> MQGSVTEFLKPRLVDIEQVSSTHAKVTLEPLERGFGHTLGNALRRILLSSMPGCAVTEVEIDGVLHEYSTKEGVQEDILEILLNLKGLAVRVQGKDEVILTLNKSGIGPVTAADITHDGDVEI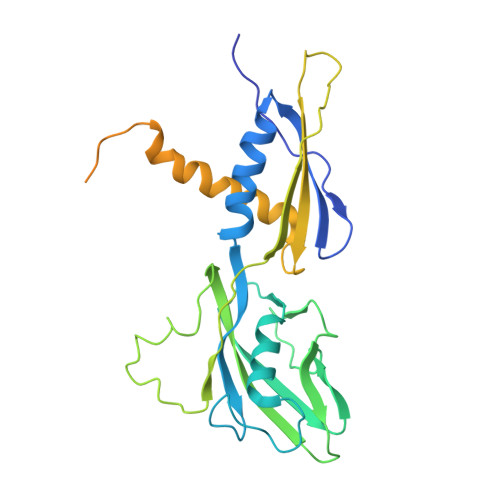VKPQHVICHLTDENASISMRIKVQRGRGYVPASTRIHSEEDERPIGRLLVDACYSPVERIAYNVEAARVEQRTDLDKLVIEMETNGTIDPEEAIRRAATILAEQLEAFVDLRDVRQPEVKEEKPEFDPILLRPVDDLELTVRSANCLKAEAIHYIGDLVQRTEVELLKTPNLGKKSLTEIKDVLASRGLSLGMRLEN> MKGMKYHDYIWDLGGTLLDNYETSTAAFVETLALYGITQD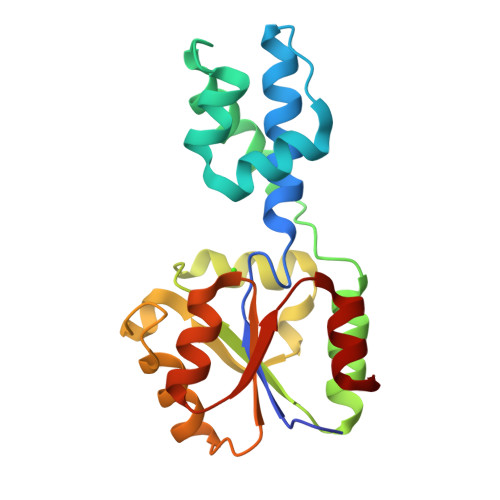HDSVYQALKVSTPFAIETFAPNLENFLEKYKENEARELEHPILFEGVSDLLEDISNQGGRHFLVSHRNDQVLEILEKTSIAAYFTEVVTSSSGFKRKPNPESMLYLREKYQISSGLVIGDRPIDIEAGQAAGLDTHLFTSIVNLRQVLDI Spiroviolene synthase (SvS) from Streptomyces violens was first described by Rabe et al. and represents a bacterial class I diterpene cyclase that we were not able to produce in sufficient quantities for crystallization due to protein instability. Terpene cyclases such as SvS form a variety of complex multicyclic compounds with potent biological activities via carbocationic, electrophilic cyclization cascades of relatively simple substrates, either by metal-ion assisted release of an allylic pyrophosphate (class I mechanism) or by protonation of an oxirane/ene-functionality (class II mechanism). We previously reported a hypothetical ancestor of SvS—SvS-A2 26—which shares 77% sequence identity with the extant enzyme.

To this aim, a small library of 24 variants of SvS-A2 was rationally designed, based on the SvS-A2 crystal structure targeting the active site as well as surrounding residues. The variants could be grouped into four categories based on their substrate preference in a Malachite Green assay: promiscuous (I), inactive (II), diterpene-specific (III), or sesquiterpene-specific (IV). One representative variant of each group was subjected to crystal structure analysis, and Cα rmsd values in the range of 0.35–0.68 Å compared to the parental SvS-A2 structure indicated that none of the variants had significant conformational rearrangements. Therefore, the altered substrate preferences are likely the consequence of steric and/or electronic interactions with substrates, intermediates and/or products, as discussed for the individual variants below. Furthermore, the studied variants were dimeric in the crystal structure and maintained a substantially elevated melting temperature similar to that of SvS-A2. A Trp156Tyr exchange (Group III) results in a highly active and diterpene specific SvS-A2 variant. The variant’s specificity for the formation of the diterpene spiroviolene over the formation of sesquiterpenes hedycaryol and farnesol can be expressed as the ratio of apparent second order rate constants and increases ca. 2.3-fold from 38.4 ± 13.7 in SvS-A2 to 88.1 ± 29.8 in the Trp156Tyr variant of SvS-A2. The exchanged position is located directly opposite of Trp79 and the introduction of Tyr may allow for additional cation-π interactions in 2, while yielding sufficient space to accommodate the bulky diterpene intermediate between Trp79 and Trp82. Alternatively, the introduced hydroxyl group may allow hydrogen bonding with residues in the adjacent effector motif. The Trp156Tyr exchange slightly reduces the melting temperature of SvS-A2 (from 71.3 ± 0.0 °C to 67.7 ± 0.1 °C) and more so of SvS-WT (from 58.2 ± 0.1 °C to 45.2 ± 0.3 °C).

>MAMTVTEVDLPPIYCPLESAIHPRVHEVEKRAVEWIRRSGMCASEEERAWVIATHSADFFARFAPTAADEDRLLATSLWVYWGFAFDDHRCDNGPLSTRPAQFNALAGRVQRALEAPSAEDNGDRFVPALQDIARRFRSFGTPTQVRRFVHAHRAYLSGVAWQIGNQARGHMPGLDDYLAMRLLSAGGEPTFAMLEIATGAEVPDREMHRPAVRALTEMAIMVAALDNDRHSLRKELSRGHTDQNIYSVLMHHRGMSLQEAVEEATKLRDRILLRFLELHDRVRPGAGAELSTYLQGLRHGIRGNAEWGLRVPRYLSLGRVPDPMEDAPLTWAESPSDSSPSPLPGAPSIAWWWDDALLGA[2x]> GPLGSMSNYSVSLVGPAPWGFRLQGGKDFNMPLT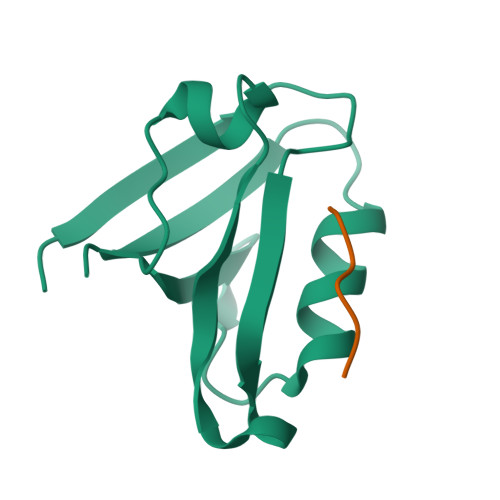ISSLKDGGKAAQANVRIGDVVLSIDGINAQGMTHLEAQNKIKGCTGSLNMTLQRAS;> DQLIDL> MSSNPHRWMMTSPGAPMVRAEFEIGELSADQVVVAVAGCGVCHTDLGYYYDSVRTNHALPLALGHEISGRVVQAGANAAQWLGRAVIVPAVMPCGTCELCTSGHGTICRDQVMPGNDIQGGFASHVVVPARGLCPVDEARLAAAGLQLADVSVVADAVTTPYQAVLQAGVEPGDVAVVIGVGGVGGYAVQIANAFGASVVAIDVDPAKLEMMSKHGAALTLN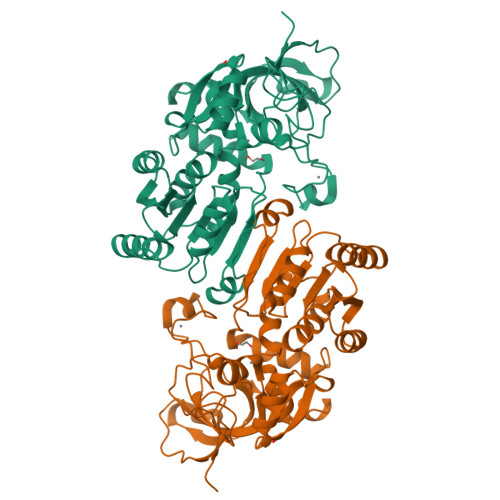AREISGRDLKKAIEAHAKANGLRLTRWKIFECSGTGAGQTSAYGLLTHGATLAVVGFTMDKVEVRLSNLMAFHARALGNWGCLPEYYPAALDLVLDAAIDLASFIERHPLDQIGEVFAAAHAHKLTRRAILTP> GLPTMNTPGSCQFLTSDDFQSPSA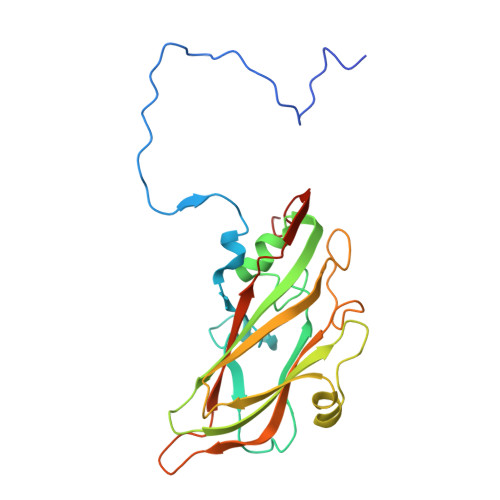MPQYDVTPEMRIPGEVKNLMEIAEVDSVVPVQNVGEKVNSMEAYQIPVRSNEGSGTQVFGFPLQPGYSSVFSRTLLGEILNYYTHWSGSIKLTFMFCGSAMATGKFLLAYSPPGAGAPTKRVDAMLGTHVVWDVGLQSSCVLCIPWISQTHYRYVTSDEYTAGGFITCWYQTNIVVPADAQSSCYIMCFVSACNDFSVRLLKDTPFISQQNFFQ2-methyl-quinolin-4(1H)-one | C10 H9 N O | 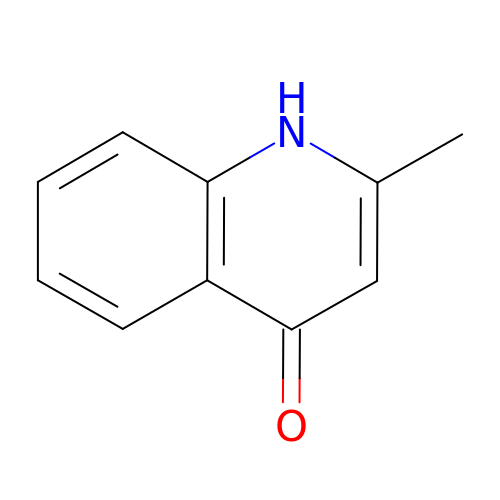NWINIEGDLHHNLH-UHFFFAOYSA-N>[2x]MHHHHHHGGDGVFKVMLLGESGVGKSTLAGTFGGLQGDNAHEMENSEDTYERRIMVDKEEVTLIVYDIWEQGDAGGWLQDHCLQTGDAFLIVFSVTD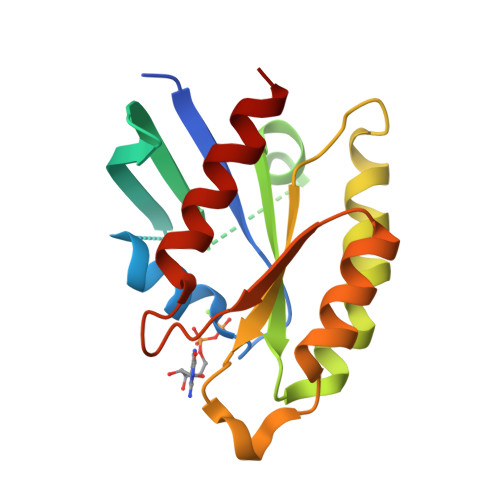RRSFSKVPETLLRLRAGRPHHDLPVILVGNKSDLARSREVSLEEGRHLAGTLSCKHIETSAALHHNTRELFEGAVRQIRLRRG>[14x]MRNGLKTYVAQTWLTLWVGLALCASSTVFSAEFATTNQLENIDFRVNKEKAAVLIVELASPSAVVDVQKVQEGLNIELLKTDVADDKLYLLDVKDFSTPVESVEVFRKAPSTQLVVTVDGEFQHDYTLKGKYLEVVISKLKADEKPKPKSVLEKEGKLISINFQDIPVRNVLQLIADYNGFNLVVSDSVVGNLTLRLDGVPWQQVLDIILQVKGLDKRVDGNVILIAPKEELDLREKQALEKARLAEELGDLKSEIIKINFAKASDIAAMIGGEGNVNMLSERGSISIDERTNSL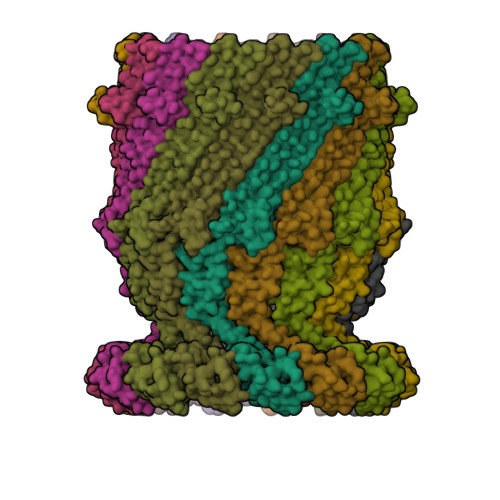LIRELPDNIAVIREIIESLDIPVKQVQIEARIVTVKEGNLEELGVRWGVMSTNGSHSVGGSIESNLWQKGLLADDEFPVDEFLNVNLASTSANASSIAFQVAKLGSGTLLDLELSALQNESKAEIISSPRLITTNKQPAYIEQGTEIPYLESSSSGASTVAFKKAVLSLKVTPQITPDNRLVLDLSVTQDRRGETVKTGTGEAVSIDTQRIGTQVLVNNGETVVLGGIFQHSINNSVDKVPLLGDLPVLGALFRRTYEQMGKSELLIFVTPKVVIQ> GGGUACUUAAGCCCACUGAUGAGUCGCUGG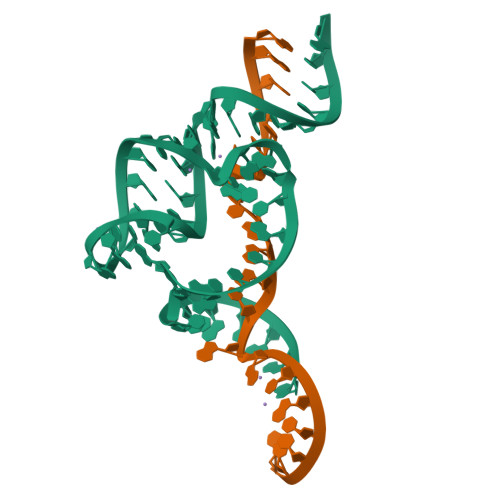GAUGCGACGAAACGCCCA;> GGGCGUCUGGGCAGUACCCA>PSVRPFKQRKSLAIRQEEVAGIRAKFPNKIPVVVERYPRETFLPPLDKTKFLVPQELTMTQFLSIIRSRMVLRATEAFYLLVNNKSLVSMSATMAEIYRDYKDEDGFVYMTYASQETF[8x];>[8x]PQQEDEWVNVQYPD

All six mATG8s are essential for autophagy, are conjugated to autophagosomes and serve to recruit two broad classes of molecules: autophagy receptors and autophagy adaptors. On the other hand, autophagy adaptor proteins interact with mATG8 proteins on the convex autophagosomal membrane surface and can regulate autophagosome formation (ULK1/2 16), autophagosome transport (FYCO1 17), crosstalk with the endocytic network (TBC1D5 18) and autophagosome fusion with the lysosome (PLEKHM1 19), but are themselves not degraded by autophagy. Structural studies have shown that the side chains of the aromatic residue (Θ) within the core LIR motif are placed deep inside of a hydrophobic pocket (HP1) on the Atg8/LC3/GABARAP surface, formed between α‐helix 2 and β‐strand 2, while side chains of the hydrophobic LIR residues (Γ) occupies a second hydrophobic pocket (HP2) between β‐strand 2 and α‐helix 3 (reviewed in 3, 23, 24). To provide a molecular basis for the specificity of the PLEKHM1‐LIR interaction with the mATG8 proteins, we solved the crystal structures of PLEKHM1‐LIR in complex with the LC3A, LC3C, GABARAP and GABARAP‐L1 proteins.

LC3C could not be crystallized as a chimeric construct, but co‐crystals of LC3C with the PLEKHM1‐LIR peptide (residues 629–642) diffracted to 2.19 Å resolution. Partner residues in each mATG8 protein are given W635 of PLEKHM1 interacts with E19 of LC3A with 3.5 Å distance, with D19 of LC3B and E25 in LC3C in similar way, but the bond distances are higher (6.2 Å and 4.5 Å), suggesting a weaker interaction. For the LC3 subfamily proteins, the hydrogen bonding distance of N637 (LIR) with K30 (LC3) correlates with binding affinity to the LIR peptide. For LC3A, two of the four monomers in the ASU do not show this interaction and in LC3C, one of the eight monomers in the ASU do not have this interaction, suggesting that this interaction is variable in the LC3 structures. In the LC3 subfamily proteins (left plot), R70/70/76 (LC3A/B/C) side chains are closer to the CG1/2 atoms of V638 (˜3.6/3.7/4.1 Å), while for GABARAP subfamily (right plot) these distances are 4.6 Å (GABARAP) and 4.2 Å (GABARAP‐L1). Due to this closer proximity, R70/70/76 polar groups become more fixed in their position and organize neighbouring negatively charged carboxyl groups of the D48/48/54 via salt bridges. V51 GABARAPs’ side chains are in close proximity to the PLEKHM1 V638 (3.8 and 4.3 Å for GABARAP and GABARAP‐L1, respectively), while side chains of residues in equivalent positions of LC3 subfamily proteins are further away (LC3A/B/C V54/V54/V60 – 4.2/4.6/4.6 Å). Similarly, GABARAPs’ L55 side chain are closer to the PLEKHM1 V638 (4.6 and 4.8 Å for GABARAP and GABARAP‐L1, respectively); LC3A/LC3B/LC3C V58/V58/L64 are distanced to PLEKHM1 V638 at 5.5/5.4/4.3 Å. Superimposition of LC3C and GABARAP‐L1 α2 helix (having biggest difference in orientation) in other projection (obtained from structures above after rotation in 90° around x‐axis).>[2x]GSHMELTPDQQTLLHFIMDSYNKQRMPQEITNKILKEAFSAEENFLILTEMATNHVQVLVEFTKKLPGFQTLDHEDQIALLKGSAVEAMFLRSAEIFNKKLPSGHSDLLEARIRNSGISDEYITPMFSFYKSIGELKMTQEEYALLTAIVILSPDRQYIKDREAVEKLQEPLLDVLQKLCKIHQPENPQHFACLLGRLTELRTFNHHHAEMLMSWRVNDHKFTPLLCEIWD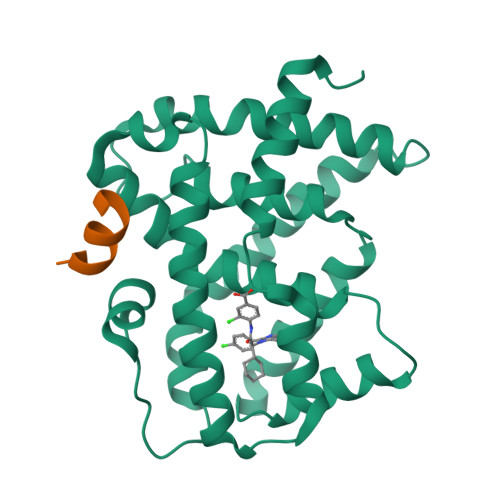VQ;>KDHQLLRYLLDKDE[2x]> TRDETSIESFLGRSGCIAM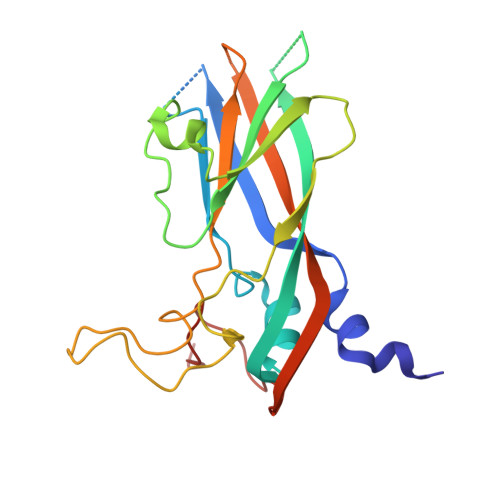IEFNTSSDKTEHDKIGKGFKTWKVSLQEMAQIRRKYELFTYTRFDSEITIVTAAAAQGNDSGHIVLQFMYVPPGAPVPEKRDDYTWQSGTNASVFWQEGQPYPRFTIPFMSIASAYYMFYDGYDGDSAASKYGSVVTNDMGTICVRIVTSNQKHDSNIVCRIYHKAKHIKAWCPRPPRAVAYQHTHSTNYIP> MATSLNTIDIQGDILVGMHKQKQLFYFFAINDPATFKTHLASDIAPVVASVTQLSNVATQPLVALNIAFSNTGLLALGVTDNLGDSLFANGQAKDATSFKESTSSWVPQFAGTGIHGVIILASDT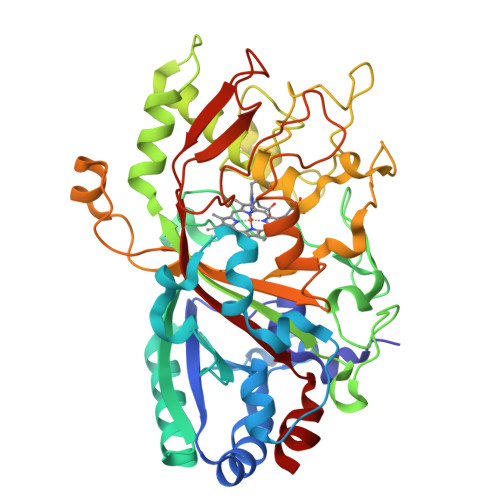TDLIDQQVASIESTFGSSISKLSSLSASIRPGNEAGHEMFGFLDLIAQPAINGFNTPLPGQNIVDAGVIITGATNDPITRPSWAVGGSFLAFRQLEQLVPEFNKYLLDNAPAGSGSLQARADLLGARMVGRWKSGAPIDLTPTADDPALGADAQRNNNFTYSHAGFDLGSDQSHCPFSAHIRKTRPRADLGGSLTPPNLSAGANSIMRSGIPYGPEVTSAESASNTTTQERGLAFVAYQAQLSQGFHFLQQTSADNANFPPGKTPATVGLDPIIGQNNGQPRVVNGLLPSNSSASLSIPQFVVSHGGEYFFSPPISAIGGRLSA> MGHHHHHHHHHHSSGHIDDDKHMVNVKKEFVDNMFSVKGKVALVTGATGALGCVLSKAYGYAG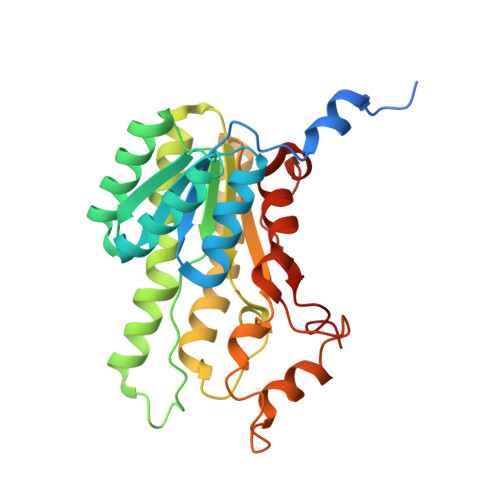AKVFMTGRNEKKLQALEAEFKAEGIDCAYGVADPADEAQVDAMITACVAQYGEVNILAVTHGFNKPQNILEQSVADWQYIMDTDCKSVYVVCKYVAQQMVDQGKGGKIVVVTSQRSKRGMAGYTGYCTSKGGADLMVSSMACDLSAKYGINVNSICPTVFRSDLTEWMFDPESAVYQNFLKREPIGRLAEPEDFVGYALFLSSDASNYITGANCDCSGGYLTC>[6x]MAILIADSGSTKTHWNVLDQGRVIGEIFTKGMNPFFQTPEEMGREIERTLLPQLNSNRFCEVHFFGAGCIPEKVPVVRNVLKGCLDVSSLIEVDTDMLAAAKASCGRSPGIVCIMGTGSNSCFYDGEKIAANVSPLGFILGDEGSGAVLGKLLIGDLLKNQMGEELKEKFLRQYELTPANIIERVYRQPFPNRFLAGISPFLAENIEHPAIHSLVLNAFKSFLTRNVMQFDYTRYKAHFIGSVAYYYKDILEEAAAATGIRTGTIVRNPMEGLRTYYSTVAKTVLEHHHHHH

Unlike other bacteria, the pathogenic Tannerella forsythia, a member of the red complex group of bacteria associated with the late stages of periodontitis, lacks biosynthetic pathways for MurNAc production and therefore obtains MurNAc from the environment. Sugar kinases play a crucial role in the MurNAc recycling process, activating the sugar molecules by phosphorylation. MurK and K1058 are two sugar kinases of the cell wall recycling system of T. forsythia, sharing a sequence identity of 44% and separated by a single PGN-scavenging operon within the genome. Structural and sequence data showed that MurK and K1058 both belong to the group of ribonuclease H-like kinases and are members of the ASKHA (acetate and sugar kinase/hsc70/actin) superfamily.

The production of MurNAc-bound crystals of MurK and K1058 was very challenging but eventually yielded crystals of MurK and K1058 in complex MurNAc (termed MurK/MurNAc and K1058/MurNAc, respectively). Both crystal forms diffract to approximately 3 Å resolution and contain six protomers in the ASU corresponding to three biological dimers. Crystals of MurK/MurNAc suffered from perfect merohedral twinning. The induced fit of MurK is triggered by binding of MurNAc into the cleft-shaped active site and results in a combined sheered rotation move of the N-terminal domain as a rigid body closing the active site over the phosphate acceptor sugar. The transition from open to closed conformation is based on helix α3, which slides over the C-terminal β-sheet towards the active site, resulting in a rotation by approximately 12° (calculated by DynDom) and a maximum translation of 6.9 Å measured for the Cα distance of residue S88 when comparing open and closed states. The anomeric carbon of the glucosamine ring of MurNAc adopts a β-configuration and is held in place by a strictly conserved catalytic residue D95 that establishes hydrogen bonding to the hydroxy groups of C4 and C6. G67 forms a hydrogen bond to the ether bond of the lactyl ether entity via its backbone amide, whereas D95, N119, and D141 utilize their side chains to recognize the hydroxy groups at atom C4 and C6, C4, and C1, respectively. The N-acetyl group dips into a rather hydrophobic cavity that is formed by the backbone of G67 and a set of three phenylalanine side chains (F34, F35, F137). No direct protein interactions are observed to account for the negative charge of the carboxyl group besides shape complementarity of the protein, predominately created by P134 on top of which the lactyl ether sits. Most obviously, residues S133, P134, and L135 in MurK allow for MurNAc binding by providing sufficient space for the lactyl ether substituent.> MHHHHHHGRMDYKDDDDKADYKDDDDKADYKDDDDKGRPMTEEVDFLGQDSDGGSEEVVLTPAELIERLEQAWMNEKFAPELLESKPEIVECVMEQLEHMEENLRRAKREDLKVSIHQMEMERIRYVLSSYLRCRLMKIEKFFPHVLEKEKTRPEGEPSSLSPEELAFAREFMANTESYLKNVALKHMPPNLQKVDLFRAVPKPDLD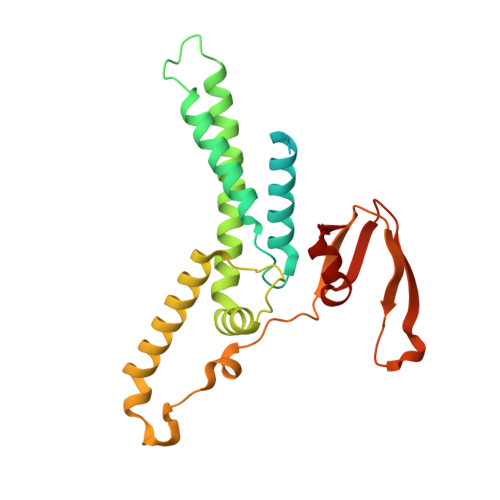SYVFLRVRERQENILVEPDTDEQRDYVIDLEKGSQHLIRYKTIAPLVASGAVQLI Here we present two crystal structures of LaIHA, one bound to the hydrolytic product isatinate, and one bound to benzyl benzoate, as well as the apo structure of homologous RsIHA. Together with results from enzyme kinetic analysis, the resolved structures are used to describe the molecular basis for the Mn2+-dependent mechanism of hydrolysis, showing that IHA is a true orthologue of IHB. The highly conserved Mn2+ binding site is located at the bottom of the substrate-binding pocket.

The structures of LaIHA:benzyl benzoate and LaIHA:isatinate were determined at 1.50 Å and 1.79 Å resolution, respectively, while the one of RsIHA was determined at 2.65 Å resolution. The more distant homolog from Ralstonia solanacearum (RsIHA) shares 59% SI with LaIHA and 51% SI with LaIHB. Unlike the whole sequence, the active site and substrate binding pocket are highly conserved among these proteins. Even though the key substrate binding pocket residues originally identified in the structure of LaIHB - Phe63, Trp65 and Trp84 and Phe20917 do not share equivalent positions in the sequences of LaIHA or RsIHA, their aromatic side chains do adopt an identical structural conformation in the respective binding pockets, thus indicating functional conservation. Compared to LaIHB, the Mn2+ binding sites in both RsIHA and LaIHA include Gln219, also responsible for increased metal specificity. Structural superposition revealed identical metal binding sites in the two homologues. Activity measurements confirm that both LaIHA and RsIHA have isatin hydrolase activity. The determination of the catalytic parameters assuming Michaelis-Menten kinetics yields Km values for LaIHA and RsIHA of 16 μM and 10 μM, respectively. The enzyme kinetics analyses, accompanying structural determination of LaIHA and RsIHA, present striking evidence that RsIHA, LaIHA, and LaIHB are true orthologues enzymes.

>AMATSTTPTILPALAAGLARGNIRVVDLTQTLSPSFPTLQLPSQFGQVQPFKIERISHYDASGPAWYWNNFSCGEHTGTHFDAPAHWITGRDYPGNSVDTIAPENFVAPAVVIDASAQVRENEDWLLTVDFLQAWEQRHGRIPAGAWVLFRTDWSLRVGDAAAFLNIREDGAHTPGPTQEAVEWLIGERNVHGFGVETINTDAGQSYAWPLAYPCHTLMHGANRYGLQCLKNLDQLPPRGAFILAAPLKIEGGSGSPLRVLALVE[10x]>MLPKLVITHRVHEEILQLLAPHCELITNQTDSTLTREEILRRCRDAQAMMAFMPDRVDADFLQACPELRVIGCALKGFDNFDVDACTARGVWLTFVPDLLTVPTAELAIGLAVGLGRHLRAADAFVRSGKFRGWQPRFYGTGLDNATVGFLGMGAIGLAMADRLQGWGATLQYHEAKALDTQTEQRLGLRQVACSELFASSDFILLALPLNADTLHLVNAELLALVRPGALLVNPCRGSVVDEAAVLAALERGQLGGYAADVFEMEDWARADRPQQIDPALLAHPNTLFTPHIGSAVRAVKLEIERCAAQNILQALAGERPINAVNRLP[2x]

Phosphite dehydrogenase (PTDH), first discovered in Pseudomonas stutzeri WM88, catalyzes the oxidation of phosphite to phosphate, which is coupled to the reduction of NAD+ to NADH. The enzyme follows an ordered kinetic mechanism with NAD+ binding before phosphite. The crystal structure of 17X-PTDH indicates that Arg301 is situated at the dimer interface, but its side chain orients inwards towards the enzyme active site. As such, Arg301 is in position to directly affect catalysis, through either electrostatic interactions if it is in the guanidinium form, or by acting as a catalytic base to deprotonate a water molecule if the guanidine is deprotonated.

In addition, X-ray crystal structures of R301A and R301K were obtained. Crystals were obtained that contained NAD+ and that diffracted to 2.35 Å and 2.65 Å for the R301A and R301K mutants, respectively. Unfortunately, the side chain of Lys301 exhibits poor electron density in the latter mutant indicating that the Lys does not occupy a well-defined position in the crystal. Although the R301K mutant possesses slightly higher activity than the parent enzyme, amine bases failed to affect the activity of the R301A mutant. Attempts to co-crystallize the PTDH mutants with sulfite inhibitor and NAD+ were unsuccessful.>GSHMASMHTVLQIGAGGVGSVVAHKMGMNRDVFKNIILASRSLDKCYAIKESMLKKGLGEIGVEQVDADDTQALVALIQKYKPKVVINVALPYQDLTIMQACLETKTHYIDTANYEHPDLAKFEYKEQWAFDRAYKEARILGVLGAGFDPGVTNAYVAHAQRHHFDTIHTLDILDCNAGDHKRPFATNFNPEINLREVSSKGRYYENGKWIETKPLEIKQVWAYPQIGEMDSYLLYHEELESLVKNIKGLRRARFFMTFSQNYLTHMKCLENVGMLGIKEIEHQGVKIVPIQFL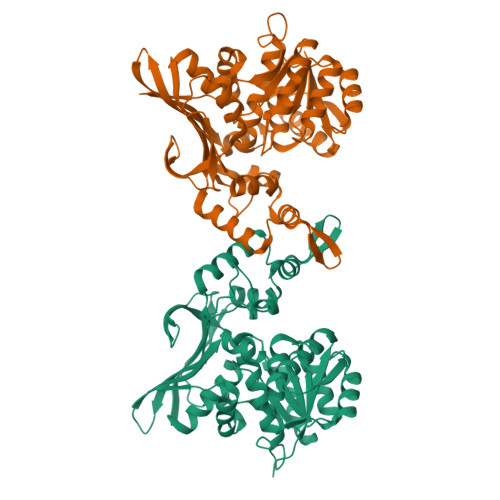KTLLPDPATLAKDTTGKTNIGCYMTGIKNNQDKTLYIYNVCDHKKCYEEVGSQAISYTTGVPAMCAAKMICNDTWSADHFRAGVFNIEELNTDPFMEELIKQGLPYEVIER[3x]>[2x]QAQITGRPEWIWLALGTALMGLGTLYFLVKGMGVSDPDAKKFYAITTLVPAIAFTMYLSMLLGYGLTMVPFGGEQNPIYWARYADWLFTTPLLALDLALLVDADQGTIL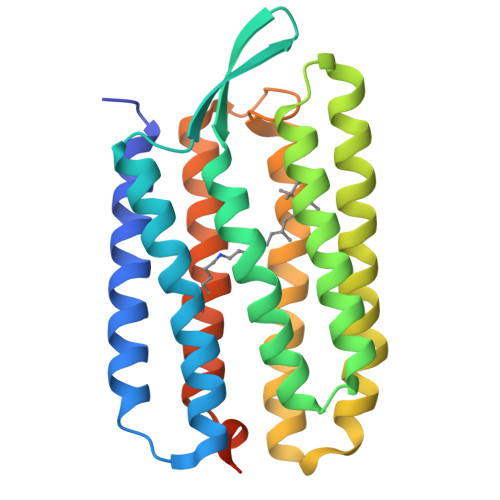ALVGADGIMIGTGLVGALTKVYSYRFVWWAISTAAMLYILYVLFFGFTSKAESMRPEVASTFKVLRNVTVVLWSAYPVVWLIGSEGAGIVPLNIETLLFMVLDVSAKVGFGLILLRSRAIFGEAEAPEPSAGDGAAATSD> KETAAA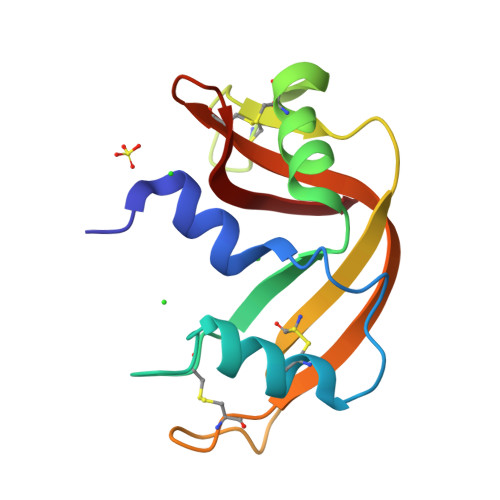KFERQHMDSSTSAASSSNYCNQMMKSRNLTKDRCKPVNTFVHESLADVQAVCSQKNVACKNGQTNCYQSYSTMSITDCRETGSSKYPNCAYKTTQANKHIIAACEGNPYVPVHFDASV>MMEQVCDVFDIYAICACCKVESKNEGKKNEVFNNYTFRGLGNKGVLPWKCISLDMKYFRAVTTYVNESKYEKLKYKRCKYLNKETVDNVNDMPNSKKLQNVVVMGRTNWESIPKKFKPLSNRINVILSRTLKKEDFDEDVYIINKVEDLIVLLGKLNYYKCFILGGSVVYQEFLEKKLIKKIYFTRINSTYECDVFFPEINENEYQIISVSDVYTSNNTTLDFIIYKKTNNKMLNEQNCIKGEEKNNDMPLKNDDKDTCHMKKLTEFYKNVDKYKINYEN[2x];>[2x]DDDDEEEDDFVYFNFNKEKEEKNKNSIHPNDFQIYNSLKYKYHPEYQYLNIIYDIMMNGNKQSDRTGVGVLSKFGYIMKFDLSQYFPLLTTKKLFLRGIIEELLWFIRGETNGNTLLNKNVRIWEANGTREFLDNRKLFHREVNDLGPIYGFQWRHFGAEYTNMYDNYENKGVDQLKNIINLIKNDPTSRRILLCAWNVKDLDQMALPPCHILCQFYVFDGKLSCIMY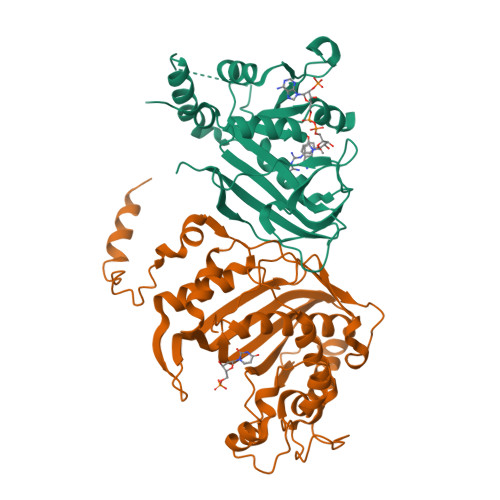QRSCDLGLGVPFNIASYSIFTHMIAQVCNLQPAQFIHVLGNAHVYNNHIDSLKIQLNRIPYPFPTLKLNPDIKNIEDFTISDFTIQNYVHHEKISMDMAA(2S)-2-amino-1-(1,3-dihydro-2H-isoindol-2-yl)-2-[(1r,4S)-4-(pyrrolidin-1-yl)cyclohexyl]ethan-1-one | C20 H29 N3 O | 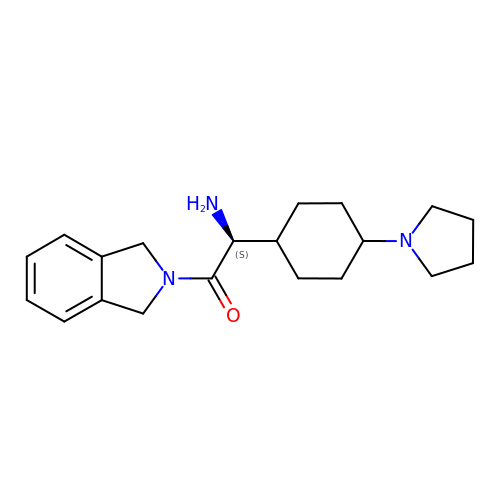SYXDQNGJEXFDND-SNRMKQJTSA-N>LP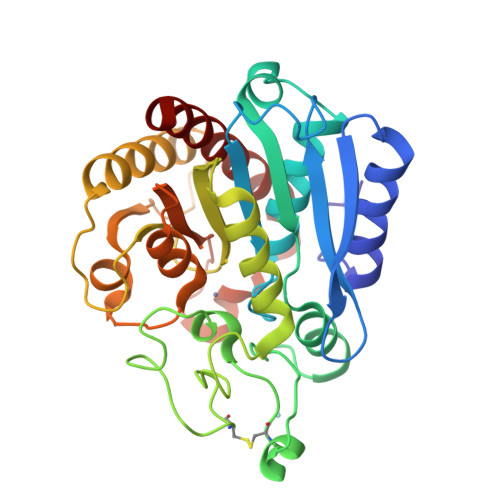YDNYQELEVIDEYLDYIGEKYPDVATVVNAAESFEGRPIKYIKISTTNFEDENKPVIFIDGGIHAREWISPPSVTWAIHKLVEDVTENDLLEKFDWILLPVVNPDGYKYTFTNERFWRKTRSTNNNPLSQICRGADGNRNFDFVWNSIGTSNSPCSDIYAGTSAFSEVETRVVRDILHEHLARMALYLTMHSFGSMILYPWGHDGSLSQNALGLHTVGVAMASVIQSNALPNFPPYTVGNSALVIGYYIAGSSEDYAHSIGVPLSYTYELPGLSSGWDGFHLPPQYIEQVCRETWEGIVVGARRAGDLFR[2x]>GCGGGCCCGC[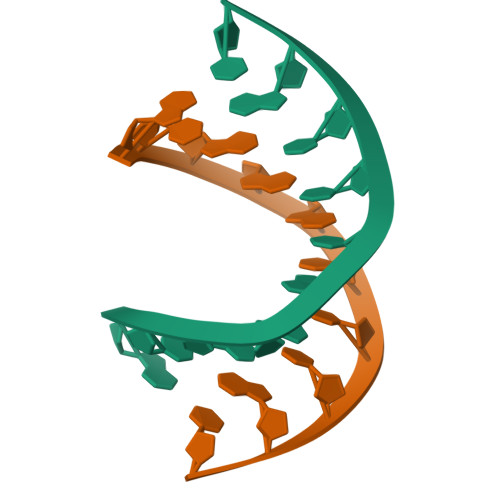2x]>[6x]PFINIKLV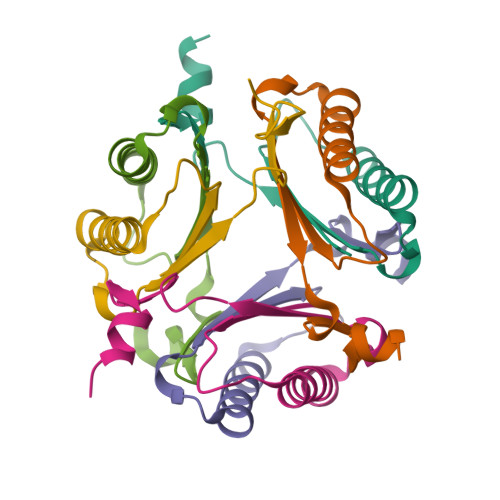PENGGPTNEQKQQLIEGVSDLMVKVLNKNKASIVVIIDEVDSNNYGLGGESVHHLRQKN3-[[(2~{R},3~{S},4~{R},5~{R})-5-[2-azanyl-7-[(3-chlorophenyl)methyl]-6-oxidanylidene-1~{H}-purin-7-ium-9-yl]-3,4-bis(oxidanyl)oxolan-2-yl]methylamino]-4-oxidanyl-cyclobut-3-ene-1,2-dione | C21 H20 Cl N6 O7 | 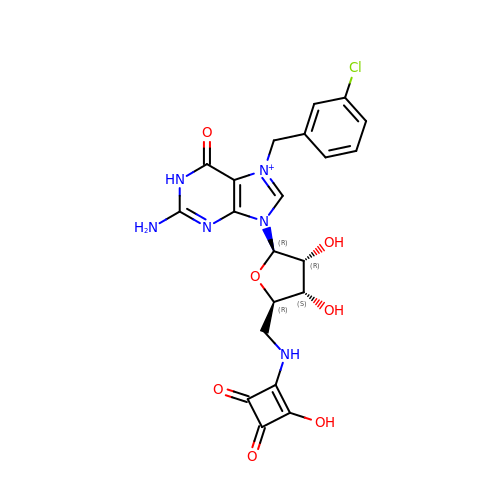IHSJKXMUPLBBMG-PRXMSPFESA-O>MSEFRIHHDVNELLSLLRVHGGDGAEVYIDLLQKNRTPYVTTTVSAHSAKVKIAEFSRTPEDFLKKYDELKSKNTRNLDPLVYLLSKLTEDKETLQYLQQNAKERAELAAAAVGSSTTSINVPAAASKISMQELEELRKQLGSVATGSTLQQSLELKRKMLRDKQNKKNSGQHLPIFPAWVYERPALIGDFLIGAGISTDTALPIGTLPLASQESAVVEDLLYVLVGVDGRYVSAQPLAGRQSRTFLVDPNLDLSIRELVHRILPVAASYSAVTRFIEEKSSFEYGQVNHALAAAMRTLVKEHLILVSQLEQLHRQGLLSLQKLWFYIQPAMRTMDILASLATSVDKGECLGGSTLSLLHDRSFSYTGDSQAQELCLYLTKAASAPYFEVLEKWIYRGIIHDPYSEFMVEEHELRKERIQEDYNDKYWDQRYTIVQQQIPSFLQKMADKILSTGKYLNVVRECGHDVTCPVAKEIIYTLKERAYVEQIEKAFNYASKVLLDFLMEEKELVAHLRSIKRYFLMDQGDFFVHFMDLAEEELRKPVEDITPPRLEALLELALRMSTANTDPFKDDLKIDLMPHDLITQLLRVLAIETKQEKAMAHADPTELALSGLEAFSFDYIVKWPLSLIINRKALTRYQMLFRHMFYCKHVERQLCSVWISNKTAKQHSLHSAQWFAGAFTLRQRMLNFVQNIQYYMMFEVMEPTWHILEKNLKSASNIDDVLGHHTGFLDTCLKDCMLTNPELLKVFSKLMSVCVMFTNCMQKFTQSMKLDGELGGQTLEHSTVLGLPAGAEERARKELARKHLAEHADTVQLVSGFEATINKFDKNFSAHLLDLLARLSIYSTSDCEHGMASVISRLDFNGFYTERLERLSAERSQKATPQVPVLRGPPAPAPRVAVTAQ[2x];>MATPDQKSPNVLLQNLCCRILGRSEADVAQQFQYAVRVIGSNFAPTVERDEFLVAEKIKKELIRQRREADAALFSELHRKLHSQGVLKNKWSILYLLLSLSEDPRRQPSKVSSYATLFAQALPRDAHSTPYYYARPQTLPLSYQDRSAQSAQSSGSVGSSGISSIGLCALSGPAPAPQSLLPGQSNQAPGVGDCLRQQLGSRLAWTLTANQPSSQATTSKGVPSAVSRNMTRSRREGDTGGTMEITEAALVRDILYVFQGIDGKNIKMNNTENCYKVEGKANLSRSLRDTAVRLSELGWLHNKIRRYTDQRSLDRSFGLVGQSFCAALHQELREYYRLLSVLHSQLQLEDDQGVNLGLESSLTLRRLLVWTYDPKIRLKTLAALVDHCQGRKGGELASAVHAYTKTGDPYMRSLVQHILSLVSHPVLSFLYRWIYDGELEDTYHEFFVASDPTVKTDRLWHDKYTLRKSMIPSFMTMDQSRKVLLIGKSINFLHQVCHDQTPTTKMIAVTKSAESPQDAADLFTDLENAFQGKIDAAYFETSKYLLDVLNKKYSLLDHMQAMRRYLLLGQGDFIRHLMDLLKPELVRPATTLYQHNLTGILETAVRATNAQFDSPEILRRLDVRLLEVSPGDTGWDVFSLDYHVDGPIATVFTRECMSHYLRVFNFLWRAKRMEYILTDIRKGHMCNAKLLRNMPEFSGVLHQCHILASEMVHFIHQMQYYITFEVLECSWDELWNKVQQAQDLDHIIAAHEVFLDTIISRCLLDSDSRALLNQLRAVFDQIIELQNAQDAIYRAALEELQRRLQFEEKKKQREIEGQWGVTAAEEEEENKRIGEFKESIPKMCSQLRILTHFYQGIVQQFLVLLTTSSDESLRFLSFRLDFNEHYKAREPRLRVSLGTRGRRSSHT[4x];>MIHELLLALSGYPGSIFTWNKRSGLQVSQDFPFLHPSETSVLNRLCRLGTDYIRFTEFIEQYTGHVQQQDHHPSQQGQGGLHGIYLRAFCTGLDSVLQPYRQALLDLEQEFLGDPHLSISHVNYFLDQFQLLFPSVMVVVEQIKSQKIHGCQILETVYKHSCGGLPPVRSALEKILAVCHGVMYKQLSAWMLHGLLLDQHEEFFIKQGPSSGNVSAQPEEDEEDLGIGGLTGKQLRELQDLRLIEEENMLAPSLKQFSLRVEILPSYIPVRVAEKILFVGESVQMFENQNVNLTRKGSILKNQEDTFAAELHRLKQQPLFSLVDFEQVVDRIRSTVAEHLWKLMVEESDLLGQLKIIKDFYLLGRGELFQAFIDTAQHMLKTPPTAVTEHDVNVAFQQSAHKVLLDDDNLLPLLHLTIEYHGKEHKADATQAREGPSRETSPREAPASGWAALGLSYKVQWPLHILFTPAVLEKYNVVFKYLLSVRRVQAELQHCWALQMQRKHLKSNQTDAIKWRLRNHMAFLVDNLQYYLQVDVLESQFSQLLHQINSTRDFESIRLAHDHFLSNLLAQSFILLKPVFHCLNEILDLCHSFCSLVSQNLGPLDERGAAQLSILVKGFSRQSSLLFKILSSVRNHQINSDLAQLLLRLDYNKYYTQAGGTLGSFGM[2x];>MARHGPPWSRLDAQQERDVRELVRGVAGLQDEADPNFQLALNFAWSNFRFHRFLDVNSHKIEKTIEGIYEKFVIHSDLSKAASWKRLTEEFLNAPLPSIKEIKTDAHYSILSLLLCLSDSPSNSSYVETPRNKEVEKKDDFDWGKYLMEDEEMDIGPYMDTPNWSEESEEENDQQPLSREDSGIQVDRTPLEEQDQNRKLDPCISWKDEPDDRSWLEHHVVHQYWTARPSQFPHSLHLHSNLAAVWDQHLYSSDPLYVPDDRVLVTETQVIRETLWLLSGVKKLFIFQLIDGKVTVRNNIIVTHLTHSCLRSVLEQIAAYGQVVFRLQEFIDEVMGHSSESMLPGSGSVPKKSTEAPFRTYQAFMWALYKYFISFKEELAEIEKCIINNDTTITLAIVVDKLAPRLSQLKVLHKVFSTGVAEVPPDTRNVVRASHLLNTLYKAILEYDNVGEASEQTVSLLFSLWVETVRPYLQTVDEWIVHGHLWDGAREFIIQRNKNVPVNHRDFWYATYTLYSVSEKTENEEKMSDNASASSGSDQGPSSRQHTMVSFLKPVLKQIIMAGKSMQLLKNLQCAESTTCQAGARDAERKSLYTLFLESVQSRLRHGEDSTPQVLTEQQATKENLMKMQSIAESHLELDDVHDPLLAINFARMYLEQSDFHEKFAGGDVCVDRSSESVTCQTFELTLRSCLYPHIDKQYLDCCGNLMQTLKKDYRLVEYLQAMRNFFLMEGGDTMYDFYTSIFDKIREKETWQNVSFLNVQLQEAVGQRYPEDSSRLSISFENVDTAKKKLPVHILDGLTLSYKVPWPVDIVISLECQKIYNQVFLLLLQIKWAKYSLDVLLFGELVSTAEKPRLKEGLIHEQDTVAQFGPQKEPVRQQIHRMFLLRVKLMHFVNSLHNYIMTRILHSTGLEFQHQVEEAKDLDQLIKIHYRYLSTIHDRCLLREKVSFVKEAIMKVLNLALMFADGWQAGLGTWRMESIEKMESDFKNCHMFLVTILNKAVCRGSFPHLESLALSLMAGMEQS[2x];> MASITQLFDDLCEALLPAAKTHLGQRSVNRKRAKRSLKKVAYNALFTNLFQDETQQLQPDMSKLPARNKILMLSFDLRVGGLGPKADRLEELVEELEAAPCCPLLEVGSVLDLLVQLAGSGPPQVLPRKRDYFLNNKHVGRNVPYSGYDCDDLSVFEMDVQSLISREECLCHSMIQETLQVMEAAPGTGLPTVGLFSFGDPCGDRFERDTRVSLFGALVHSRTYDMDVRLGLPPVPDNADLSGLAIKVPPSVDQWEDEGFQSASNLTPDSQSEPSVTPDVDLWEAALTYEASKRRCWERVGCPPGHREEPYLTEAGRDAFDKFCRLHQGELQLLAGGVLQAPQPVLVKECELVK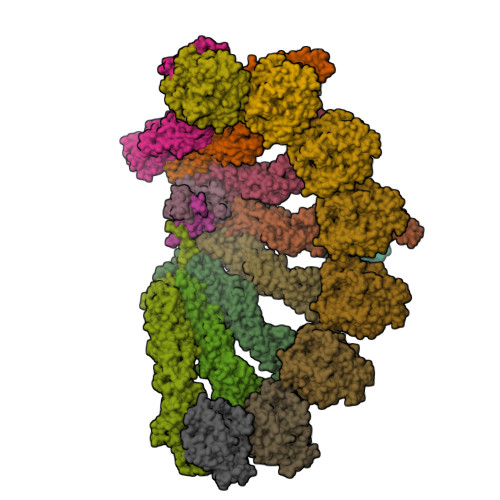DVLNVLIGVVSATFSLCQPAQAFVVKRGVHVSGASPESISSLLSEVAEYGTCYTRLSHFSLQPVLDSLYSKGLVFQAFTSGLRRYLQYYRACVLSTPPTLSLLTIGFLFKKLGRQLRYLAELCGVGAVLPGTCGGGPRAAFPTGVKLLSYLYQEALHNCSNEHYPVLLSLLKTSCEPYTRFIHDWVYSGVFRDAYGEFMIQVNHEYLSFRDKLYWTHGYVLISKEVEDCVPVFLKHIAHDIYVCGKTINLLKLCCPRHYLCWSDVPVPRISVIFSLEELKEIEKDCAVYVGRMERVARHSSVSKEEKELRMEIAKQELIAHAREAASRVLSALSDRQMSERMALDARKREQFQRLKEQFVKDQERRQAARQEELDDDFSYARELRDRERRLKSLEEELERKARQALVDHYSKLSAEAARREQKALWRIQRHRLESARLRFLLEDEKHIQEMLKAVSEAHQPQEPPDVLLSVHPQVTSPGPEHPEGGQGCDSGSAEQHSPAWDGWNRPGLLTPQPLKPLAVGAGGRGLQQAEGARPFSDSLSIGDFLPVGPGAEPSVQTGMVPLLEVALQTINLDLPPSAPGEAPAAASTQPSRPQEYDFSTVLRPAVATSPAPGPLQAAECSLGSSGLQLWEDSCGKMDACGSASRETLLPSHPPRRAALEEGSSQPTERLFGQVSGGGLPTGDYASEIAPTRPRWNTHGHVSDASIRVGENVSDVAPTQPRWNTHGHVSNASISLGESVSDVAPTRPRWNIHGHVSNASIRVGENVSDVAPTRPRWNTHGHVSNASIRVGENVSDVAPTRPRWNTHGHVSDASISLGESVSDMAPARPRWNTHGHVSDASISLGESVSDMAPTRPRWNTHGHVSDTSIRVGENVSDVAPIRSRCNTHGHVSDASISLGEPVSDVVSTRPRWNTHVPIPPPHMVLGALSPEAEPNTPRPQQSPPGHTSQSALSLGAQSTVLDCGPRLPVEVGPSLSSPSSGCGEGSISVGENVSDVAPTQPWWPNTPGDSVSEELGPGRSGDTEDLSPNWPLNSQEDTAAQSSPGRGEEAEASAAEAQGGEQAYLAGLAGQYHLERYPDSYESMSEPPIAHLLRPVLPRAFAFPVDPQVQSAADETAVQLSELLTLPVLMKRSITAPLAAHISLVNKAAVDYFFVELHLEAHYEALRHFLLMEDGEFAQSLSDLLFEKLGAGQTPGELLNPLVLNSVLSKALQCSLHGDTPHASNLSLALKYLPEVFAPNAPDVLSCLELRYKVDWPLNIVITEGCVSKYSGVFSFLLQLKLMMWALKDVCFHLKRTALLSHMAGSVQFRQLQLFKHEMQHFVKVIQGYIANQILHVTWCEFRARLATVGDLEEIQRAHAEYLHKAVFRGLLTEKAAPVMNVIHSIFSLVLKFRSQLISQAWGPPGGPRGAEHPNFALMQQSYNTFKYYSHFLFKVVTKLVNRGYQPHLEDFLLRINFNNYYQDA;>[8x]MPREIITLQLGQCGNQIGFEFWKQLCAEHGISPEGIVEEFATEGTDRKDVFFYQADDEHYIPRAVLLDLEPRVIHSILNSPYAKLYNPENIYLSEHGGGAGNNWASGFSQGEKIHEDIFDIIDREADGSDSLEGFVLCHSIAGGTGSGLGSYLLERLNDRYPKKLVQTYSVFPNQDEMSDVVVQPYNSLLTLKRLTQNADCVVVLDNTALNRIATDRLHIQNPSFSQINQLVSTIMSASTTTLRYPGYMNNDLIGLIASLIPTPRLHFLMTGYTPLTTDQSVASVRKTTVLDVMRRLLQPKNVMVSTGRDRQTNHCYIAILNIIQGEVDPTQVHKSLQRIRERKLANFIPWGPASIQVALSRKSPYLPSAHRVSGLMMANHTSISSLFERTCRQYDKLRKREAFLEQFRKEDMFKDNFDEMDTSREIVQQLIDEYHAATRPDYISWGTQEQ;>[3x]MASSSGAGAAAAAAAANLNAVRETMDVLLEISRILNTGLDMETLSICVRLCEQGINPEALSSVIKELRKATEALKAAENMTS> MDAKEFREFGKAAIDYIADYLENIRDDDVLPNVEPGYLLDLLPTEMPEEPEAWKDVLGDISRVIKPGLTHWQSPHMHAYYPTSTSYPSIVGEMLASGFGVIGFSWICSPACTELEVVVMDWLAKFLKLPAHFQHASDGPGGGVIQGSASEAVLVAVLAAREQAVANYRESHPELSESEVRGRLVAYSSDQSNSCIEKAGVLAAMPIRLLPAGEDFVLRGDTLRGAIEEDVAAGRIPVICVATLGTTGTCAYDDIESLSAVCEEFKVWLHVDAAYAGGAFALEECSDLRKGLDRVDSLNFNLHKFMLVNFDCSAMWLRDANKV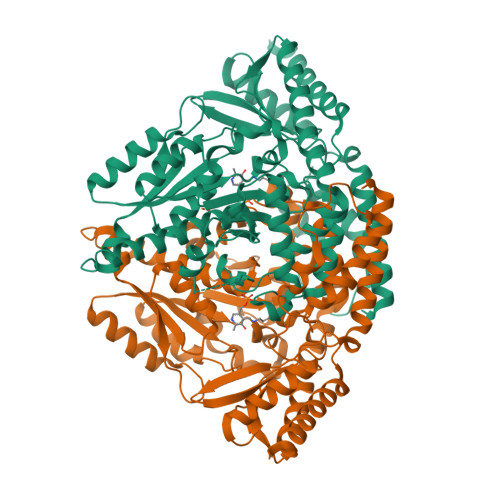VDSFNVDRIYLKHKHEGQSQIPDFRHWQIPLGRRFRALKVWITFRTLGAEGLRNHVRKHIELAKQFEQLVLKDSRFELVAPRALGLVCFRPKGDNEITTQLLQRLMDRKKIYMVKAEHAGRQFLRFVVCGMDTKASDIDFAWQEIESQLTDLQAEQSLVARKSGNVGDLAQHFQIHLSTENATHEKSQ>SMAHLTMPYVMPGDGEVVGVGEPVAIRFDENIADRGAAEKAIKITTNPPVEGAFYWLNNREVRWRPEHFWKPGTAVDVAVNTYGVDLGEGMFGEDNVQTHFTIGDEVIATADDNTKILTVRVNGEVVKSMPTSMGKDSTPTANGIYIVGSRYKHIIMDSSTYGVPVNSPNGYRTDVDWATQISYSGVFVHSAPWSVGAQGHTNTSHGCLNVSPSNAQWFYDHVKRGDIVEVVNTVGGTLPGIDGLGDWNIPWD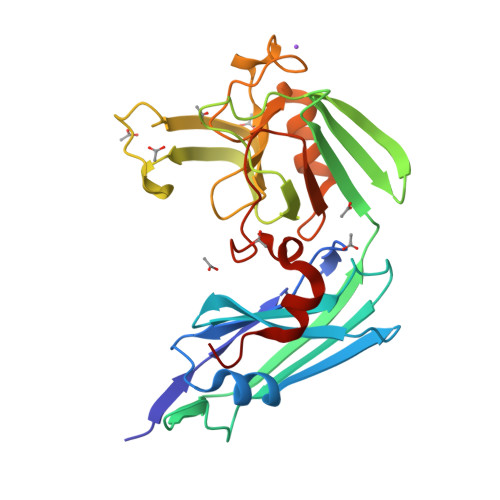QWRAGNAKA[2x]Eukaryotes possess eight highly conserved Lsm (like Sm) proteins that assemble into circular, heteroheptameric complexes, bind RNA, and direct a diverse range of biological processes. Among the many essential functions of Lsm proteins, the cytoplasmic Lsm1–7 complex initiates mRNA decay, while the nuclear Lsm2–8 complex acts as a chaperone for U6 spliceosomal RNA. The Sm family includes the Sm, Lsm (“Like Sm”), and bacterial Hfq proteins. These proteins share a conserved “Sm fold” consisting of an amino-terminal alpha helix followed by five antiparallel beta strands that form small beta barrels that assemble into ring-shaped hexamers or heptamers. Here, we elucidate the molecular basis for Lsm-RNA recognition and present four high-resolution structures of Lsm complexes bound to RNAs.

We crystallized the Lsm2–8 complex bound to UUUUU-3′-OH and UUUUU > p and determined their structures by X-ray diffraction to resolutions of 1.9 and 2.3 Å, respectively. In the Lsm2–8 complex bound to the UUUUU-3′-OH RNA, the 5′ uridine is bound by Lsm4, and the next three uridines are bound sequentially by Lsm8, Lsm2, and Lsm3. Uridine binding involves stacking and an extensive hydrogen bonding network as previously described (Zhou et al. 2014a; Montemayor et al. 2018). The last uridine with the 3′-OH group is disordered except for its 5′ phosphate as evidenced by weak electron density for both the ribose and uracil groups. We confirmed that the RNA remains completely intact after prolonged incubation with Lsm2–8, further supporting the idea that the last uridine is covalently attached but disordered in the structure. Consistent with this, Lsm2–8 still binds to oligoU RNA ending in 3′-OH, with a Kd of 100 nM. For example, Lsm2–8 binds to telomerase RNA (TER1), which has a stretch of 3–6 uridines ending with a 3′-OH.

>[2x]MLFYSFFKTLIDTEVTVELKNDMSIRGILKSVDQFLNVKLENISVVDASKYPHMAAVKDLFIRGSVVRYVHMSSAYVDTILLADACRRDLANNKRQ;>[2x]GSMESAQAVAEPLDLVRLSLDEIVYVKLRGDRELNGRLHAYDEHLNMVLGDAEEIVTIFDDEETDKDKALKTIRKHYEMLFVRGDSVILIAPPRN;>[2x]MLPLTLLNATQGRPILVELKNGETFNGHLENCDNYMNLTLREVIRTMPDGDKFFRLPECYIRGNNIKYLRIQDEVLSQVAKQQAQQRENRGSRFRGRGQRGRGNYGHTAPNRRGRGRGGHMWSHPQFEK;>MSMTILPLELIDKCIGSNLWVIMKSEREFAGTLVGFDDYVNIVLKDVTEYDTVTGVTEKHSEMLLNGNGMCMLIPGGKPE[2x];>[2x]GSMDSSPNEFLNKVIGKKVLIRLSSGVDYKGILSCLDGYMNLALERTEEYVNGKKTNVYGDAFIRGNNVLYVSALDD;>[2x]MSSLQKRPGPGNSSQPTERPRKESILDLSRYQDQRIQATFTGGRQITGILKGFDQLMNLVLDDVEEQLRNPEDGKLTGAIRKLGLVVVRGTTLVLIAPMDGSEEIPNPFVQAEHHHHHH;>[2x]MSLADFMEQRVQVITNDGRVVLGSLKGFDHTTNLILSDSFERIISMDQDMETIPLGVYLLRGENVAMVGLVNEELDSEIEWTKIRGEAIPDVVH benzyl (carboxyoxy)carbamate | C9 H9 N O5 | 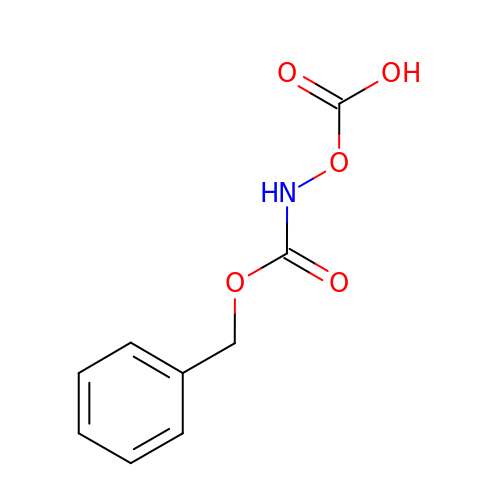DUVYLXOFESFFPT-UHFFFAOYSA-N>MAHHHHHHMNAVSEALKRTAIDPSIKVDGKRLWNSLMEMAKIGATPKGGVCRLALTDLDKAGRDLIVRWAKEAGCTVTVDTMGNVFMRRAGRVADAAPVVTGSHADSQPTGGRFDGIYGVLGGLEVIRSLNDHGIETEHPIEVVIWTNEEGSRFAPAMVASGVFAGVFTLEYGLSRKDVDGKTIGEELQRIGYAGDVPCGGRPLHAAFELHIEQGPILEAERKTIGVVTDAQGQRWYEITFTGQEAHAGPTPMPRRRDALLGASRVVDLVNRIGLDHAPFGCATVGMMQVHPNSRNVIPGRVFFTVDFRHPDDAVLAQMDAALRDGVARIAADIGLETALEQIFYYKPVAFDPACVQAVREAAERFGYPHRDIVS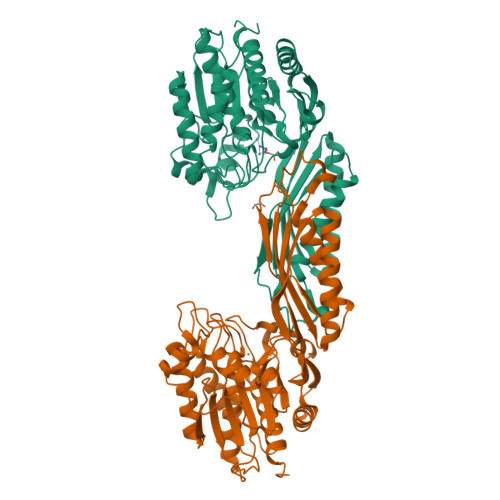GAGHDACYLAQVAPTSMVFVPCVDGISHNEVEDATPEWIEAGANVLLHAMLSRACEPVS[4x]> MAGLNDIFEAQKIEWHELEVLFQGPMSPDVVLVNGGEPPNPLIPTGTNDSNGGRIIDRLFAGLMSYDAVGKPSLEVAQSIESADNVNYRITVKPGWKFTDGSPVTAHSFVDAWNYGALSTNAQLQQHFFSPIEGFDDVAGAPGDKSRTTMSGLRVVNDLEFTVRLKAPTIDFTLRLGHSSFYPLPDSAFRDMAAFGRNPIGNGPYKLADGPAGPAWEHNVRIDLVPNPD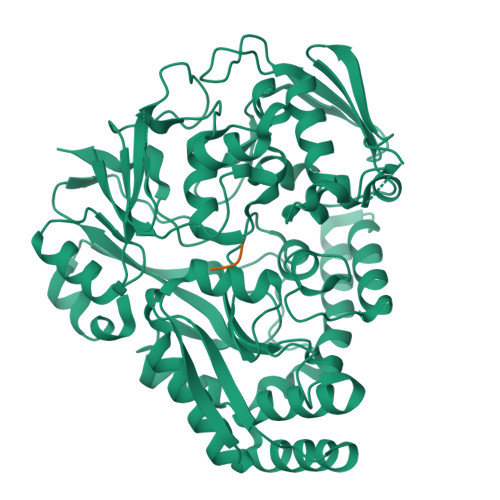YHGNRKPRNKGLRFEFYANLDTAYADLLSGNLDVLDTIPPSALTVYQRDLGDHATSGPAAINQTLDTPLRLPHFGGEEGRLRRLALSAAINRPQICQQIFAGTRSPARDFTARSLPGFDPNLPGNEVLDYDPQRARRLWAQADAISPWSGRYAIAYNADAGHRDWVDAVANSIKNVLGIDAVAAPQPTFAGFRTQITNRAIDSAFRAGWRGDYPSMIEFLAPLFTAGAGSNDVGYINPEFDAALAAAEAAPTLTESHELVNDAQRILFHDMPVVPLWDYISVVGWSSQVSNVTVTWNGLPDYENIVKAENLYFQGGHHHHHHHH;> SVA> SNAMLYPLLTKTRNTYDLGGIWNFKLGEHNPNELLPSDEVMVIPTSFNDLMVSKEKRDYIGDFWYEKVIEVPKVSEDEEMVLRFGSVTHQAKIYVDGVLVGEHKGGFTPFEVLVPECKYNNEKIKVSICANNVLDYTTLPVGNYSEIIQEDGSIKKKVRENFDFFNYAGVHRPLKLMIRPKNHIFDITITSRLSDDLQSADLHFLVETNQKVDEVRISVFDEDNKLVGETKDSRLFLSDVHLWEVLNAYLYTARVEIFVDNQLQDVYEENFGLREIEVTNGQFLLNRKPIYFKGFGKHEDTFINGRGLNEAANLMDLNLLKDMGANSFRTSHYPYSEEMMRLADRMGVLVIDEVPAVGLFQNFNASLDLSPKDNGTWNLMQTKAAHEQAIQELVKRDKNHPSVVMWVVANE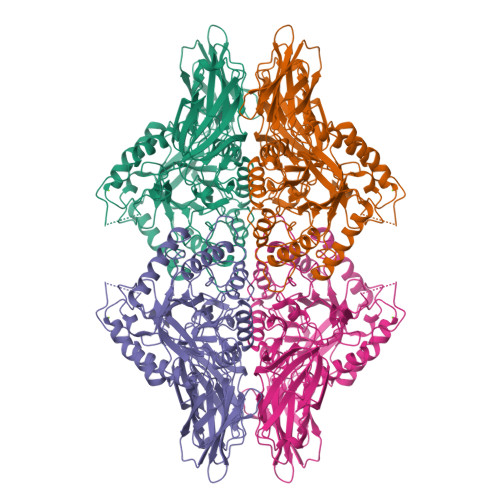PASHEAGAHDYFEPLVKLYKDLDPQKRPVTLVNILMATPDRDQVMDLVDVVCLNRYYGWYVDHGDLTNAEVGIRKELLEWQDKFPDKPIIITEYGADTLPGLHSTWNIPYTEEFQCDFYEMSHRVFDGIPNLVGEQVWNFADFETNLMILRVQGNHKGLFSRNRQPKQVVKEFKKRWMTIPHYHNKKNSVK The B cell adaptor protein (BCAP) is a multimodular regulator of inflammatory signaling in diverse immune system cells. BCAP couples TLR signaling to phosphoinositide metabolism and inhibits MyD88-directed signal transduction. BCAP is recruited to the TLR signalosome forming multitypic interactions with the MAL and MyD88 signaling adaptors. Using a combination of biophysical and structural techniques, we show that dimerization of BCAP TIR by the DBB domain drives negative regulation of TLR signaling.

Subsequently, the shorter TIG2α construct was crystallized, and the structure was solved at 3.1 Å using data from a native crystal and phases from a selenomethionine derivative. Data collection, phasing, and refinement statistics are summarized in Supplemental Table I. The DBB domain structure reveals a typical TIG fold followed by two α helices. The TIG domain is composed of seven β-strands (βA–βG) that make up a C-type Ig fold with a broken βA strand. The DBB TIG fold exhibits structural similarity to TIG domains from several TFs despite low sequence similarity. It shares an identical domain topology with the NFAT, NF-κB, CAMTA, and Ebf1 TIG domains, with root-mean-square deviation (RMSD) values as low as 1.6 Å (21–24). The TIG dimerization interface in TF is composed of symmetrical interactions of the ABED β-sheet. The conformation of these TF dimers shares a high level of similarity to one of the crystal contacts in the TIG2α structure with RMSD values as low as 2.3 Å. This finding strongly indicates that the crystal contacts in the BCAP TIG2α crystal represent the physiological dimerization interface, even though TIG2α is monomeric in solution. The TIG2α dimer also shares the helical features of the Ebf1 structure. By contrast, a DBB construct lacking the last C-terminal α helix (TIG2α, residues 179–288) was monomeric in solution.

>[5x]SNAMVVQPDRIRCGAETTVYVIVRCKLDDRVATEAEFSPEDSPSVRMEAKVENEYTISVKAPNLSSGNVSLKIYSGDLVVCETVISYYTDMEEIGNLLSNAANPVEFMCQAFK>MGFWGLEVKPGKPQAYNPKNEQGKIHVTQATLGTGLSKEKSVIQCSIGDKAPIALCSLLPNKIECCPLNLEFDDDDEPVEFTVTGDRSIHLSGFLEYYQ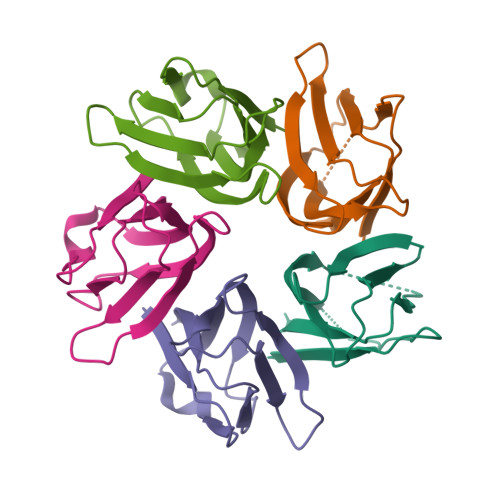DLEHHHHHH[10x]> MELI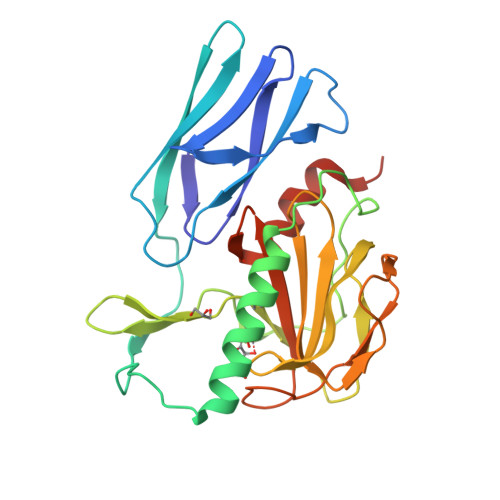KGQALFLELDKKDFLSLKNNDKNIPTFAHPKNQEKILAIFSLPYKNPPQNTKLIAFYKDKKEEIFIKTLEGNYKSEKLQVENKKIFPPKTIQERIAKELKEANAIYSSYTPKALFNGAFNIPLNSFITSDFGKARTFNEKVASYHSGTDFRAATGTPIYAANSGVVKIAKDRYFAGNSVVIDHGFGIYSQYYHLSKIDVKVGQKIKKGELIGLSGASGRVSGPHLHFGILAGGKQVDPLDFVSKFNAIFQLEHHHHHH>[2x]MSSTTRDVSHL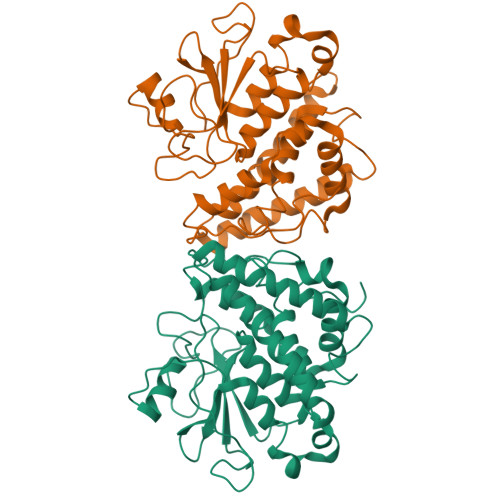SDISKSISEPDGSFNRKPSVFRNFVEKGGAFAPEKGRYHLYVSYACPWATRTLIVRKIKGLEEFIDVSVVSPRMGAHGWPFANVDAFPGADADPLFGAEHVKDLYMRVNPDYEGRFTVPILWDKKTSAIVNNESSEIIRMFNTAFNDQLPSDKAAIDLYPEALRGEIDGINEWVYDTVNNGVYKSGFATSQKAYEAAVVPLFESLDRLEKILTGKDYLVGDQLTEADIRLFVTIVRFDPVYVGHFKCNIRTIRDGYPAIDLWMRKLYWNNSAFSSTCNFEHIKTHYYWSHPQINPHRVVPVGPIPNILPLHHHHHH> HHHHHHHMPITINNFRYSDPVNNDTIIMMEPPYCKGLDIYYKAFKITDRIWIVPERYEFGTKPEDFNPPSSLIEGASEYYDPNYLRTDSDKDRFLQTMVKLFNRIKNNVAGEALLDKIINAIPYLGNSYSLLDKFDTNSNSVSFNLLEQDPSGATTKSAMLTNLIIFGPGPVLNKNEVRGIVLRVDNKNYFPCRDGFGSIMQMAFCPEYVPTFDNVIENITSLTIGKSKYFQDPALLLMAQLIAVLHGLYGMQVSSHEIIPSKQEIYMQHTYPISAEELFTFGGQDANLISIDIKNDLYEKTLNDYKAIANKLSQVTSCNDPNIDIDSYKQIYQQKYQFDKDSNGQYIVNEDKFQILYNSIMYGFTEIELGKKFNIKTRLSFFSMNHDPVKIPNLLDDTIYNDTEGFNIESKDLKSEYKGQNMRVNTNAFRNVDGSGLVSKLIGLCKKIIPPTNIRENLYNRTASLTDLGGELCIKIKNEDLTFIAEKNSFSEEPFQDEIVSYNTKNKPLNFNYSLDKIIVDYNLQSKITLPNDRTTPVTKGIPYAPEYKSNAASTIEIHNIDDNTIYQYLYAQKSPTTLQRITMTNSVDDALINSTKIYSYFPSVISKVNQGAQGILFLQWVRDIIDDFTNESSQKTTIDKISDVSTIVPYIGPALNIVKQGYEGNFIGALETTGVVLLLEYIPEITLPVIAALSIAESSTQKEKIIKTIDNFLEKRYEKWIEVYKLVKAKWLGTVNTQFQKRSYQMYRSLEYQVDAIKKIIDYEYKIYSGPDKEQIADEINNLKNKLEEKANKAMININIFMRESSRSFLVNQMINEAKKQLLEFDTQSKNILMQYIKANSKFIGITELKKLESKINKVFSTPIPFSYSKNLDCWVDNEEDIDVILKKSTILNLDINNDIISDISGFNSSVITYPDAQLVPGINGKAIHLVNNESSEVIVHKAMDIEYNDMFNNFTVSFWLRVPKVSASHLEQYGTNEYSIISSMKKHSLSIGSGWSVSLKGNNLIWTLKDSAGEVRQITFRDLPDKFNAYLANKWVFITITNDRLSSANLYINGVLMGSAEITGLGAIREDNNITLKLDRCNNNNQYVSIDKFRIFCKALNPKEIEKLYTSYLSITFLRDFWGNPLRYDTEYYLIPVASSSKDVQLKNITDYMYLTNAPSYTNGKLNIYYRRLYNGLKFIIKRYTPNNEIDSFVKSGDFIKLYVSYNNNEHIVGYPKDGNAFNNLDRILRVGYNAPGIPLYKKMEAVKLRDLKTYSVQLKL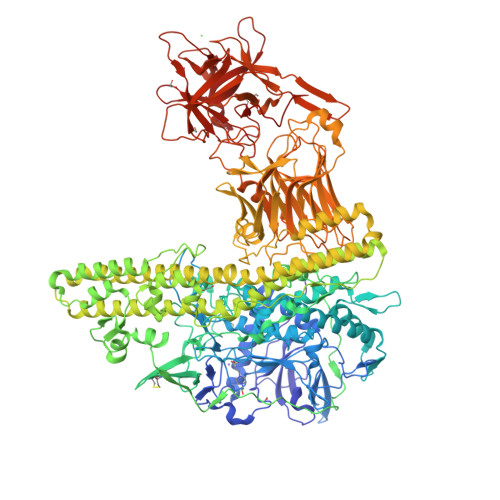YDDKNASLGLVGTHNGQIGNDPNRDILIASNWYFNHLKDKILGCDWYFVPTDEGWTND> MGFEFTLMVVGESGLGKSTLVNSLFLTDLYPERIIPDAIEKQKQTVKLEASTVEIEERGVKLRLTVVDTPGFGDAIDNSNSFGAILEYIDEQYERFLRDESGLNRRNIVDNRIHCCFYFISPFGHGLKPLDVEFMKKL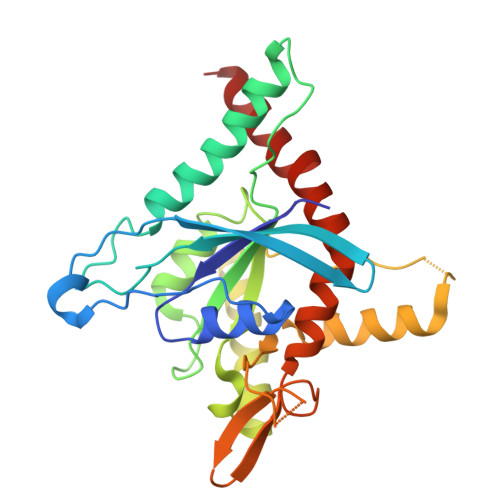HSKVNIVPVIAKADCLTKKEILRLKCRIMQEIESHGIKIYPLPDCDSDEDEDYKEQVKQLKEAVPFAVCGANTLLEVKGKKVRGRLYPWGVVEVENPDHCDFIKLRTMLITHMQDLQEVTQEVHYENYRSDRLAKGI>SG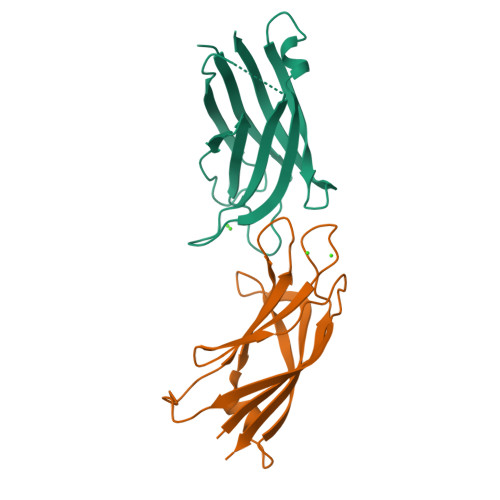GGGGMLRVFILYAENVHTPDTDISDAYCSAVFAGVKKRTKVIKNSVNPVWNEGFEWDLKGIPLDQGSELHVVVKDHETMGRNRFLGEAKVPLREVLATPSLSASFNAPLLDTKKQPTGASLVLQVSYTPLPGAVL[4x]>[2x]EQQVNV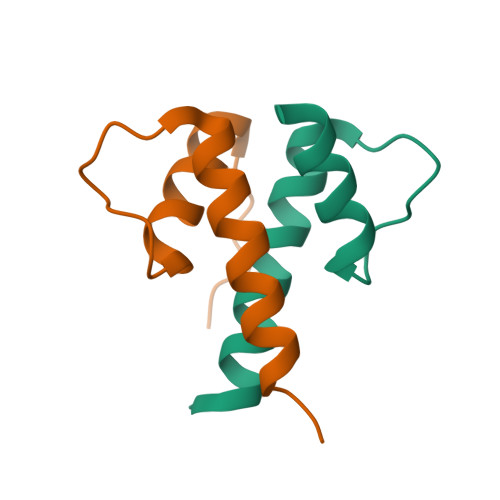LLYDMNGCYSRLKELVPTLPQNRKVSKVEILQHVIDYIRDLQLELNS(5S)-3,5-bis(4-chlorobenzyl)-4-(6-chloro-1H-indol-3-yl)-5-hydroxy-1-methyl-1,5-dihydro-2H-pyrrol-2-one 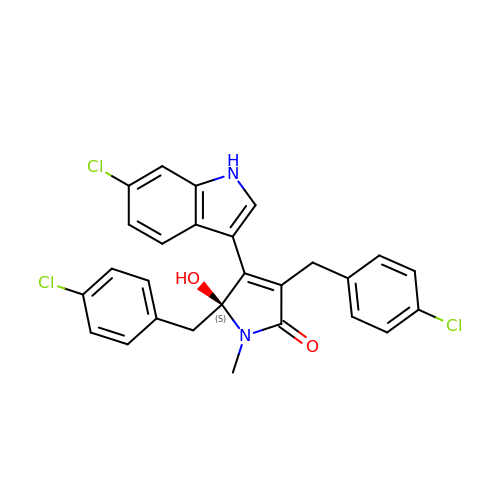| C27 H21 Cl3 N2 O2 | HHGSWONIEYVVCX-MHZLTWQESA-N>[2x]MRGSHHHHHHGSMPQYKLTYFDIRGLGEGARLIFHQAGVKFEDNRLKREDWPALKPKTPFGQLPLLEVDGEVLAQSAAIYRYLGRQFGLAGKTPMEEAQVDSIFDQFKDFMAEL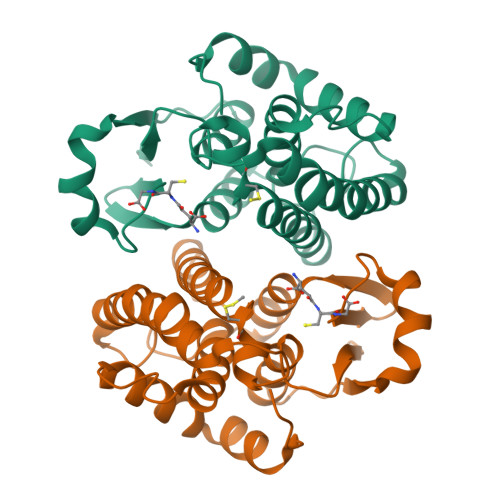RPCFRVLAGFEEGDKEKVLKEVAVPARDKHLPLLEKFLAKSGSEYMVGKSVTWADLVITDSLASWESLIPDFLSGHLQLKKYIEHVRELPNIKKWIAERPKTPY> GHPGHLKGREIGLWYAKKQGQKNKEAERQERAVVHMDERREEQIVQLLHSVQTKNDKDEEAQISWFAPEDHGYGTEAYIDRDSEYLLQENEPDATLDQQLLEDLQKKKTDLRYIEMQRFREKLPSYGMQKELVNMIDNHQVTVISGETGCGKTTQVTQFILDNYIERGKGSACRIVCTQPRRISAISVAERVAAERAESCGNGNSTGYQIRLQSRLPRKQGSILYCTTGIILQWLQSDPHLSSVSHIVLDEIHERNLQSDVLMTVVKDLLSYRPDLKVVLMSATLNAEKFSEYFGNCPMIHIPGFTFPVVEYLLEDIIEKIRYVPEQKEHRSQFKKGFMQGHVNRQEKYYYEAIYKERWPGYLRELRQRYSASTVDVVEMMDDEKVDLNLIAALIRYIVLEEEDGAILVFLPGWDNISTLHDLLMSQVMFKSDKFIIIPLHSLMPTVNQTQVFKRTPPGVRKIVIATNIAETSITIDDVVYVIDGGKIKETHFDTQNNISTMSAEWVSKANAKQRKGRAGRVQPGHCYHLYNSLRASLLDDYQLPEILRTPLEELCLQIKILRLGGIAHFLSRLMDPPSNEAVLLSIKHLMELNALDKQEELTPLGVHLARL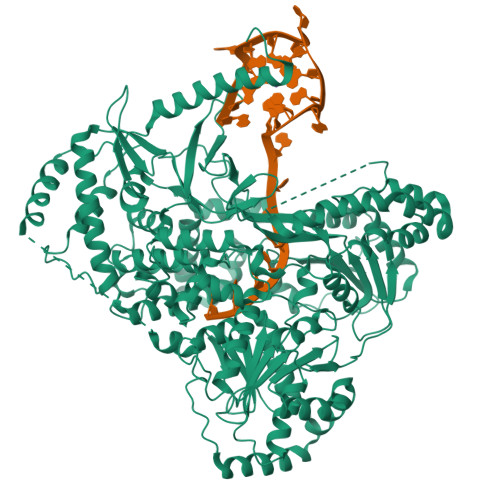PVEPHIGKMILFGALFCCLDPVLTIAASLSFKDPFVIPLGKEKVADARRKELAAATASDHLTVVNAFKGWEKAKQRGFRYEKDYCWEYFLSSNTLQMLHNMKGQFAEHLLGAGFVSSRNPQDPESNINSDNEKIIKAVICAGLYPKVAKIRLNLGKKRKMVKVYTKTDGVVAIHPKSVNVEQTEFNYNWLIYHLKMRTSSIYLYDCTEVSPYCLLFFGGDISIQKDNDQETIAVDEWIIFQSPARIAHLVKELRKELDILLQEKIESPHPVDWKDTKSRDCAVLSAIIDLIKTQEKATPRNLPPRFQDGYYSPHHHHHHHH> KHLPEPFRIRVIEPVKRTTRAYREEAIIKSGMNPFLLDSEDVFIDLLTDSGTGAVTQSMQAAMMRGDEAFSGSRSYYALAESVKNIFGYQYTIPTHQGRGAEQIYIPVLIKKREQEKGLDRSKMVAFSNYFFDTTQGHSQINGCTVRNVYIKEAFDTGVRYDFKGNFDLEGLERGIEEVGPNNVPYIVATITSNSAGGQPVSLANLKAMYSIAKKYDIPVVMDSARFAENAYFIKQREAEYKDWTIEQITRETYKYADMLAMSAKKDAMVPMGGLLCMKDDSFFDVYTECRTLCVVQEGFPTYGGLEGGAMERLAVGLYDGMNLDWLAYRIAQVQYLVDGLEEIGVVCQQAGGHAAFVDAGKLLPHIPADQFPAQALACELYKVAGIRAVEIGSFLLGRDPKTGKQLPCPAELLRLTIPRATYTQTHMDFIIEAFKHVKENAANIKGLTFTYEPKVLRHFTAKLKEV

E. coli tryptophanase (tryptophan indole-lyase, Trpase, EC 4.1.99.1) is a pyridoxal 5'-phosphate (PLP)-dependent enzyme that catalyses α,β-elimination and β-replacement reactions of L-tryptophan. Trpase consists of four identical subunits (~52 kD per monomer), each of which covalently binds one molecule of PLP. The tetramer possesses a D2 symmetry, therefore it is a dimer of dimers with two different dimeric interfaces: a catalytic interface and a non-catalytic interface. Using kinetic spectrophotometric methods and size-exclusion chromatography we have previously shown that the inactivation process is linked to the cleavage of the PLP-Lys270 aldimine bond and to the dissociation of the tetrameric form of Trpase into dimers.

The two apo mutants of E. coli Trpases as well as the wt Trpase are found in an open conformation, different than that of the closed one found for P. vulgaris in its holo form. In the Y74F mutant, the observed loss of activity at 25°C is presumably attributed to the proximity of residue 74 to the substrate binding site. In the wt Trpase the hydroxyl group of Tyr74 is hydrogen bonded to both Arg103 (at a 2.9 Å distance), and to the phosphate group of PLP (of the neighbouring subunit in the catalytic dimer) through a bridging water molecule. Replacing Y74 by phenylalanine eliminated the hydrogen bonds of the hydroxyl group thereby reducing its affinity towards PLP. Hence, the Y74F mutant exhibited negligible activity compared to the other Trpases. The Y74F mutant has low activity at 25°C and its residual activity was further reduced by cooling. It should be noted that mutant Y74F dissociates even at 25°C (about 17%). Unless the concentration of PLP is higher than 5 mM, Y74F exists as a mixture of holo and apo forms which affects the dimer-tetramer equilibrium. The catalytic dimer (AB) is further stabilized by two hydrogen bonds between the hydroxyl groups of Tyr74 and Tyr307 from one subunit to the phosphate group of the PLP molecule from the neighboring subunit.> MSEAPKKRWYVVQAFSGFEGRVATSLREHIKLHNMEDLFGEVMVPTEEVVEIRGGQRRKSERKFFPGYVLVQMVMNDASWHLVRSVPRVMGFIGGTSDRPAPISDKEVDAIMNRLQQVGDKPRPKTLFEPGEMVRVNDGPFADFNGVVEEVDYEKSRLK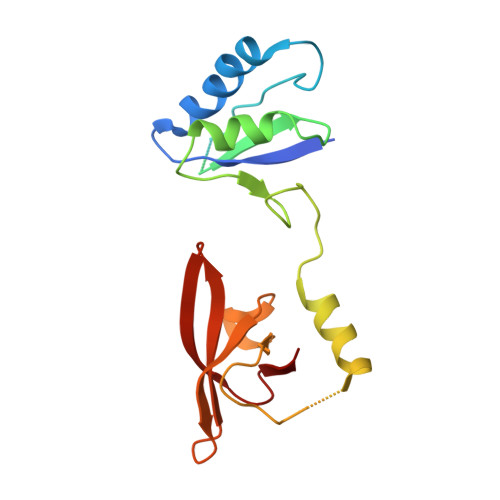VSVSIFGRATPVELDFSQVEKA>[4x]MA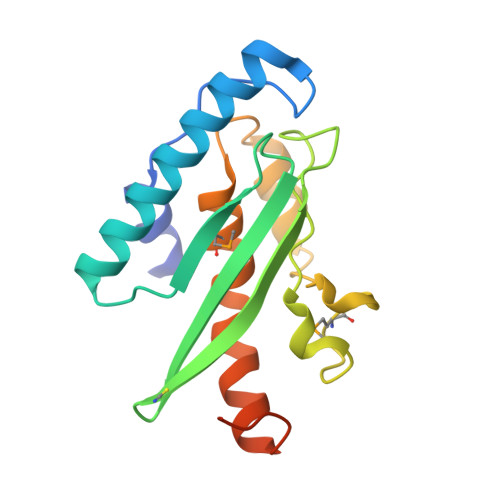DEATRRVVSEIPVLKTNAGPRDRELWVQRLKEEYQSLIRYVENNKNADNDWFRLESNKEGTRWFGKCWYIHDLLKYEFDIEFDIPITYPTTAPEIAVPELDGKTAKMYRGGKICLTDHFKPLWARNVPKFGLAHLMALGLGPWLAVEIPDLIQKGVIQHKEKCNQLEHHHHHH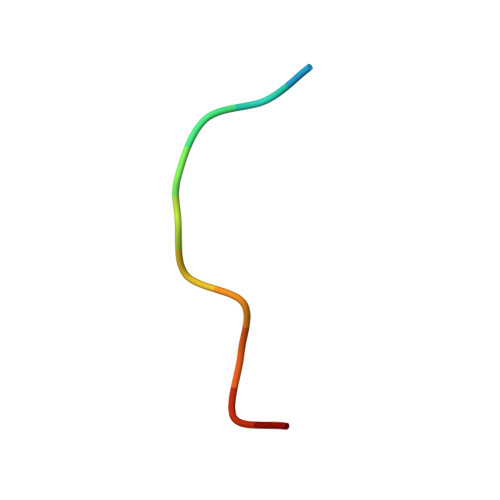> QEEEGAGGGQGG> GSMVEATAQETDRPRFSFSIAAREGKARTGTIEMKRGVIRTPAFM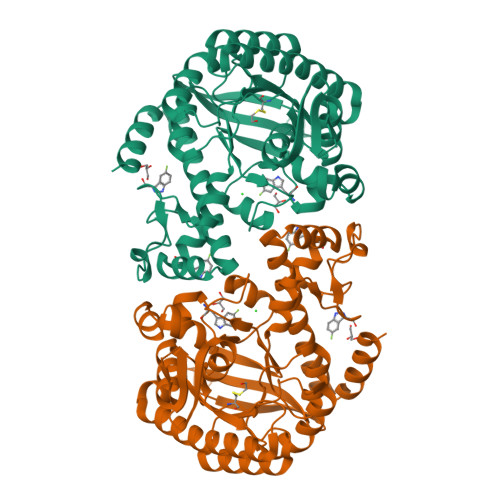PVGTAATVKALKPETVRATGADIILGNTYHLMLRPGAERIAKLGGLHSFMGWDRPILTDSGGYQVMSLSSLTKQSEEGVTFKSHLDGSRHMLSPERSIEIQHLLGSDIVMAFDECTPYPATPSRAASSMERSMRFAKRSRDAFDSRKEQAENAALFGIQQGSVFENLRQQSADALAEIGFDGYAVGGLAVGEGQDEMFRVLDFSVPMLPDDKPHYLMGVGKPDDIVGAVERGIDMFDCVLPTRSGRNGQAFTWDGPINIRNARFSEDLKPLDSECHCAVCQKWSRAYIHHLIRAGEILGAMLMTEHNIAFYQQLMQKIRDSISEGRFSQFAQDFRARYFARNS> EKVFEEPEEFLKHSQADHLLDEKGKAQSLLQREVVQSLEQQLELEKEKLGAMQAHLAGKMALAKAPSVASMDKSHGNSSFPEFFHNMDYFKYHNMRPPFTYATLIR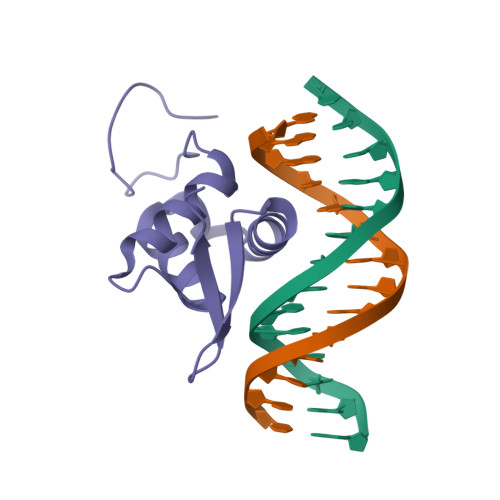WAILEAPERQRTLNEIYHWFTRMFAYFRNHPATWKNAIRHNLSLHKCFVRVESEKGAVWTVDEFEFRKKR>[2x]DPNAKENLIPEDPNED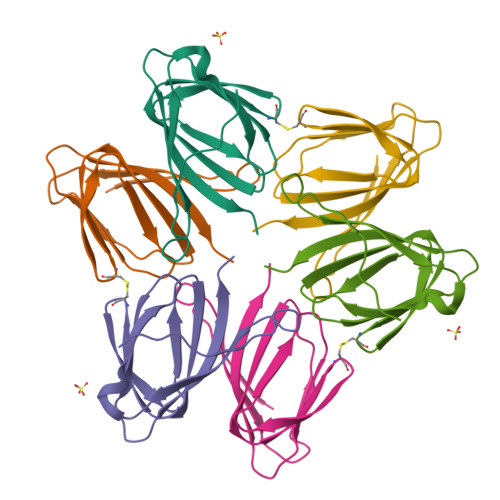IIERIESGGIENGEWLKHGILEANVKISDTKEETKDEIIAFAPNLSQTEQVKDTKDENFALEIMFDKHKEYFASGILKLPAISGQKKLSNSFRTYITFHVIQGIVEVTVCKNKFLSVKGSTFQIPAFNEYAIANRGNDEAKMFFVQVTVS>[2x]MPATDTLSLSASEALARRRSVRAFTDRPVDRALLARIFEIAQRAPSGGNLQPWQATVVTGERWQAVQDAVAARIVMGREGFQPEYDIYPRGLTDPWDSRRFGVGEALYASLGIARDDKAGRIAQFQQNYRGFGAPVMLFLHCSRIMGPPQWADMGMWLQSVMLLLVEHGLASCPQECWAMYGATVRAELGLGDDQILFSGLAIGHADEEAPVNRWPVPRVGLDEVIDWQGFDA

Recently, the nitroreductase NfnB from Sphingopyxis sp. strain HMH exhibited metabolic activity for dinitroaniline herbicides including butralin and pendimethalin, triggering the initial steps of their degradation and detoxification. The homodimer NfnB is a member of the PnbA subgroup of the nitroreductase family. Each monomer displays a central α + β fold for the core domain, with a protruding middle region and an extended C-terminal region. The protruding middle region of Val75–Tyr129 represents a structural extension that is a common feature to members of the PnbA subgroup and functions as an opening wall connecting the coenzyme FMN-binding site to the surface, therefore serving as a substrate binding site.

We determined the crystal structure of NfnB in the presence of coenzyme FMN at a resolution of 2.1 Å. Two monomers in the asymmetric unit are related by noncrystallographic twofold symmetry, with a buried surface area of 7006 Å2, calculated using the PISA analysis. Coenzyme FMN is bound to the pocket in the dimeric interface, with an opening to the surface. Within the pocket, coenzyme FMN is oriented with its isoalloxazine ring packed against the β3 backbone atoms and exposed to solvent via the opening to the surface. Arg18, Ser20, Arg22, and Arg219 mediate interactions within 3.3 Å along the ribityl moiety as follows: Arg22 to O2 of the moiety, Ser20 to O3, and Arg18, Ser20, and Arg219 all to the phosphate group of the moiety. Except for a contribution by Met180 from η4, the opening wall consists mainly of side chains of residues in the protruding middle region, including Ile87, Tyr88, Arg100, Phe101, Val103, Leu107, Tyr108, and Phe125. Near the entrance, the opening has ∼16 Å of Cα atoms between Tyr88 and Phe125 and a similar distance between Glu176 and Val103. In the structure of NfnB, Tyr88 and Arg100 are neighboring residues at an entrance to the opening and show possible interaction between their side chains within ∼3.5 Å. This observation is applicable to only one specific monomer; in the other monomer, the swung-out conformation of Arg100 forms crystallographic packing interactions with a crystallographic symmetry-related Asp26. Consistent with the findings of a previous study, butralin was the best substrate for the wildtype NfnB, followed by pendimethalin, showing 21-fold lower enzyme efficiency (kcat/Km) than butralin, whereas no activity was observed against oryzalin or isopropalin.>GSSGSSGSSSGKPGPTVIKVQNMPFTVSIDEILDF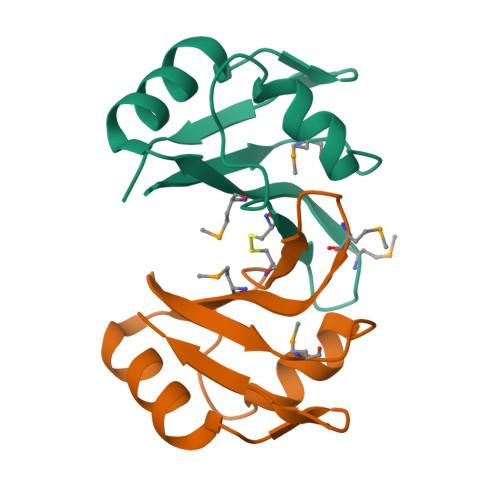FYGYQVIPGSVCLKYNEKGMPTGEAMVAFESRDEATAAVIDLNDRPIGSRKVKLSGPSSG[8x]> LSRVAK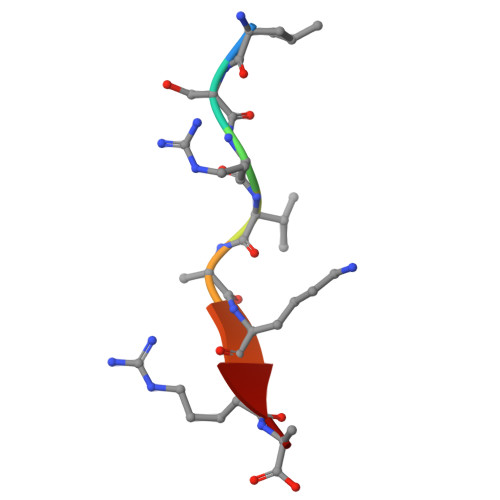RA> YCTLSSGFTTVDISMAVGRVVVRPSDPVGKILRKATFPINPNGSTLRCTSYSDTITAALTQNYPLSPLGNSIYSTNIPGIGIRLYEEAENATNFSGYYPYTRSLTPGTTYN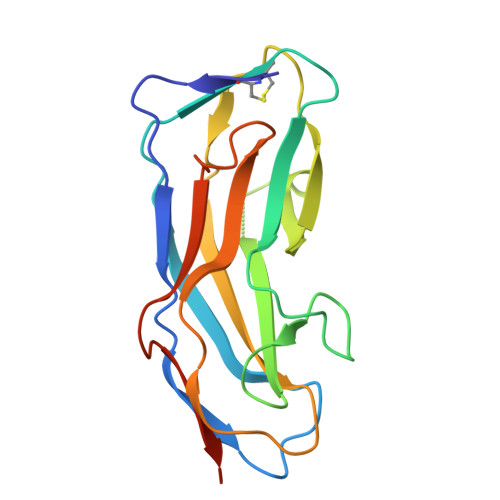LAQGYFVVEIVKTADQTGSGTLVPGLYSRYYVNGHMDRPFLTSTVYGNAITIASSSHHHHHH> NYLDQGALNNESGRSLYRKQTERVIQEEESKKVFMIINSFGGSVGNGITVHDALQFIKAGSLTL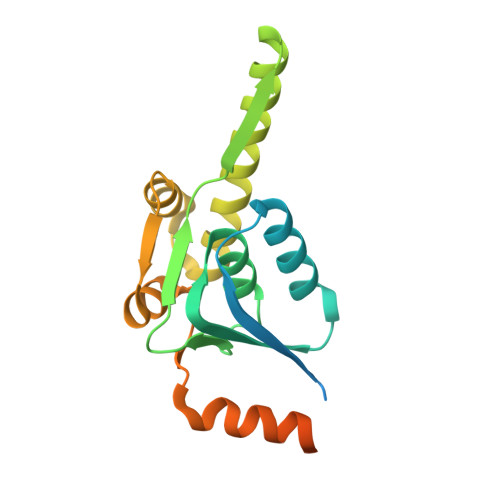ALGVAASAASLALAGGTIGERYVTEGCHTMIHQPEGGLNGQASDIWIDSQEIMKIRLDVAEIYSLSTYRPRHKILRDLDRDFYLTAMETIYYGLADEIATNEVMHSIVEMTNQVWSYHDSKQERLLESRASLVGDSTQTQESNS>MNTTPVHALTDIDGGIAVDPAPRLAGPPVFGGPGNAAFDLAPVRSTGREMLRFDFPGVSIGAAHYEEGPTGATVIHIPAGARTAVDARGGAVGLSGGYDFNHAICLAGGAGYGLEAGAGVSGALLERLEYRTGFAELQLVSSAVIYDFSARSTAVYPDKALGRAALEFAVPGEFPQGRAGAGMSASAGKVDWDRTEITGQGAAFRRLGDVRILAVVVPNPVGVIVDRAGTVVRGNYDAQTGVRRHPVFDYQEAFAEQVPPVTQA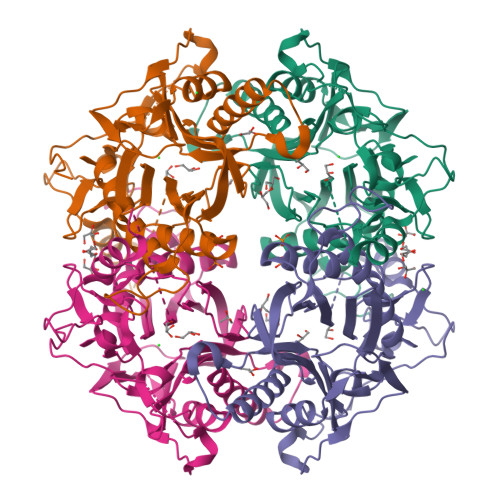GNTTISAIVTNVRMSPVELNQFAKQVHSSMHRGIQPFHTDMDGDTLFAVTTDEIDLPTTPGSSRGRLSVNATALGAIASEVMWDAVLEAGK[2x]>RRATDTTPPTITVPSDIIAYRGEEFEFYFEITDDSGQVKNIELSTFGKPLGLNWLEYSEDNFNVPGNATSDNPLRVRVHGTVPLNEPIPADKNRAQFTRTIRAWDAAGNVSSNITFVIKYRAQTDKYNPADPTITYVDRLSSLSPSE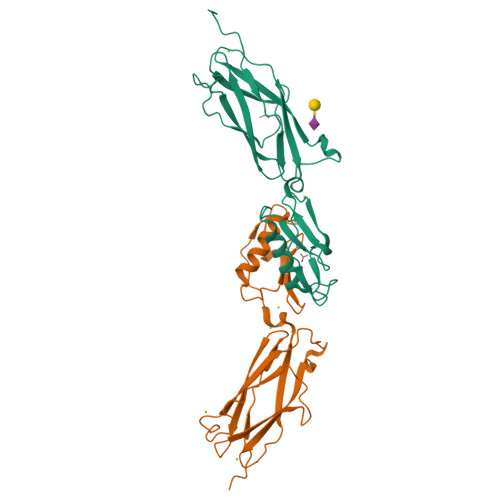KNAVEAAVRAANPQIPAAARITVSANGTVTITYPDSSTDTITANRVVKDLASS[2x]Herein, we design metalloglycosidases by constructing a hydrolytically active Zn-binding site within a barrel-shaped outer membrane protein OmpF. We supposed that a protein containing a void space, such as β-barrel outer membrane protein F (OmpF), would be suitable for our study; its overall shape resembles the structure of host compounds, such as cyclodextrin, which may provide a structural basis for various functions, including catalysis, by encompassing guest molecules and forming noncovalent interactions. We inspected the constriction zone of OmpF, the narrowest region, approximately halfway inside the barrel-shaped protein. A coordinatively unsaturated mononuclear Zn-binding site, a common catalytic motif in metallohydrolases, was created by placing three metal-coordinating histidines.

As a result, two triple mutants, R82H/Y102H/R132H (OmpF1) and L83H/Y102H/R132H (OmpF2), were designed as the parent templates. After protein extraction, purification, and refolding, they were isolated as β-barrel trimers, retaining the native overall architecture of OmpF. More importantly, both proteins possess a mononuclear Zn-binding site in the constriction zone. In OmpF1, two designed residues, R82H and R132H, coordinated to Zn ion, as expected. Consequently, OmpF1 possesses a coordinatively unsaturated Zn-site, satisfying the prerequisite for metal-dependent hydrolysis. Due to the E71 binding, the Y102H mutation becomes no longer needed for Zn coordination, while the residue may still influence the chemical properties of the Zn-site. Of note, the empty coordination site of OmpF2 pointed toward the periplasmic side, whereas that of OmpF1 is placed toward the extracellular region. In particular, D113 shows proper orientation and interatomic distance between the terminal oxygen atom and Zn-bound exchangeable ligands as 7.9–9.5 Å and 4.7–5.1 Å in OmpF1 and OmpF2, respectively.

>[3x]MAEIYNKDGNKVDLYGKAVGLHYFSKGNGENSYGGNGDMTYARLGFKGETQINSDLTGYGQWEYNFQGNNSEGADAQTGNKTHLAFAGLKYADVGSFDYGRNHGVVYDALGYTDMLPEFGGDTAYSDDFFVGHVGGVATYRNSNFFGLVDGLNFAVQYLGKNERDTARRSNGDGVGGSISYEYEGFGIVGAYGAADRTNLQEAQPLGNGKKAEQWATGLKYDANNIYLAANYGETRNATPITNKFTNTSGFANKTQDVLLVAQYQFDFGLRPSIAYTKSKAKDVEGIGDVDLVNYFEVGATYYFNKNMSTYVDYIINQIDSDNKLGVGSDDTVAVGIVYQF>[2x]MHHHHHHGRGSMETGKSDVLDKIEKINKKDSALQEIIPKGYEIEHHQCGIALNQLIPSKKEGEPDKKVFITSTIPQITERFEDIESNEVSFNMLFYDNKTPVN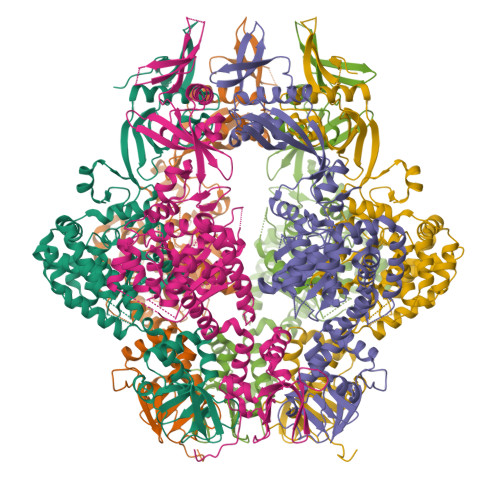IAVSAEEISDSRQLLKLVNKKLDVTSSTSTKLVDYINASKRYNPPLNVKVATRLGHVKGYFIYPYQEVMKDSNVKLFSNDKGFQKLIDSFRSKGTLQGYSKKVFAQIKDLPMVMVMLYASLGSVLLREFGLQPFIVEISGSTSTGKTFTLNLVSSVWGTSDLITTWSSTQNSIESMASFLNSFPMFKDDTRNTHPKFVTSATYNFSSGESKSRSNINLTLNAKKEWRNILISTGESSIANMADEKAGVSARVVTLQDPPYPDNFDFTTLDKSFRENYGTLGLAFIKQYESKKDVYKNAFESYQRYFNQKGSNEIMQRLGRAFALLQVTGEVLNDIDGFEHDHFKIIEQAYDSMVKNNKTIDKPKQLLEELLQYLDANRNNIAGDGYSSVKNGDIKAIYKRDYLCILGETVKEKLTHELQTITGQWDKKGYLIKGEKDRLQKQVKHQTVKYRGFAIKQEVLKELGFDFSNSYNPNSNY Ferroptosis suppressive protein 1 (FSP1) is one of the main regulators that negatively regulates ferroptosis through the GPX4‐independent FSP1–CoQ10–NAD(P)H axis and is a potential therapeutic target for ferroptosis‐related diseases. Unlike GPX4, which primarily functions in the cytoplasm and mitochondria, FSP1 localizes to mitochondria‐associated membranes (MAMs) 29 and exerts antiferroptotic effects as a coenzyme Q10 (CoQ10) oxidoreductase. 26 FSP1 reduces CoQ10 to its antioxidant form, ubiquinol, which subsequently acts as a lipid peroxidation scavenger within the mitochondrial membrane. Similar to other flavoprotein oxidoreductases, 34 , 35 the overall structure of hFSP1 comprised two tandem Rossmann fold domains (RFD) and a C‐terminal domain.

In this study, we reported the crystal structure of hFSP1 containing FAD and NADH at a resolution of 1.75 Å, which is the highest resolution structure of FSP1 to date and will benefit drug development targeting FSP1. Only one molecule of hFSP1 is present in the asymmetry unit. The two RFDs include 6‐hydroxy‐flavin adenine dinucleotide (FAD) and nicotinamide adenine dinucleotide (reduced from, NADH), and the C‐terminal domain is responsible for substrate binding, which will be discussed later. The interactions between 6‐hydroxy‐FAD and hFSP1 arise mainly from the contribution of hydrogen bonds and hydrophobic interactions. While adenine interacts with V82 and S250, isoalloxazine interacts with A295, Y296, and K355. The hydrogen bonds found between the two phosphate groups and F21, G22, and D285 further contribute to the interaction of 6‐hydroxy‐FAD and hFSP1. Hydrogen‐bond interactions also appear to be the driving force for the interaction of NADH and hFSP1. The main chains of S175 and V209 are capable of hydrogen bonding with adenine, while the main chain of L329 stabilizes nicotinamide through hydrogen bonds. E156 is conserved and forms a salt bridge with K355, which stabilizes the hydrogen bond between the C4‐carbonyl of the isoalloxazine ring and the Nζ of K355. Y296 and F360 together clamp the quinone group of CoQ, and mutagenesis of Y296 and F360 disrupted the activity of hFSP1.

> MGSQVSVESGALHVVIVGGGFGGIAAASQLQALNVPFMLVDMKDSFHHNVAALRASVETGFAKKTFISYSVTFKDNFRQGLVVGIDLKNQMVLLQGGEALPFSHLILATGSTGPFPGKFNEVSSQQAAIQAYEDMVRQVQRSRFIVVVGGGSAGVEMAAEIKTEYPEKEVTLIHSQVALADKELLPSVRQEVKEILLRKGVQLLLSERVSNLEELPLNEYREYIKVQTDKGTEVATNLVILCTGIKINSSAYRKAFESRLASSGALRVNEHLQVEGHSNVYAIGDCADVRTPKMAYLAGLHANIAVANIVNSVKQRPLQAYKPGALTFLLSMGRNDGVGQISGFYVGRLMVRLTKSRDLFVSTSWKTMRQSPP>[3x]MKQKLLVTLLGLSALGASPVFAANTNVDLAEDAYIYGYSIDEAYKFFYHTAVENNYPLNEFQNRRALADDSYTAHPTINNDTLHLMGWLDVAAEPVIVSVPDMDEGRYWILHTMDMGHYTNAAFSSRTRGTKGGQFMFAAQDWQGEVPASVDEVV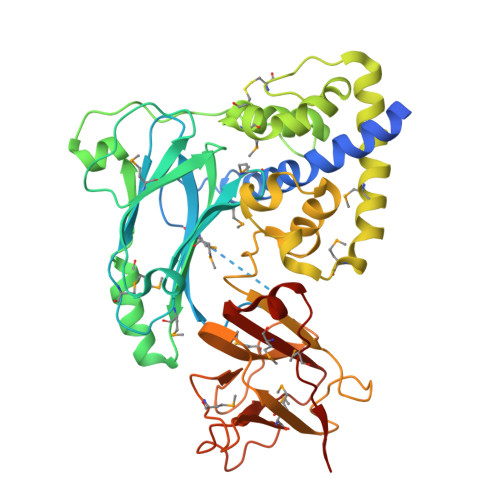RVDSNLVKLMGRIMAVNDEDAKVALNYMDQWNIRTLSEYLGKNGPKPVQRTYPDPKKSTWLERVNFVLCDGSMGNADKQWLDKYQSIGVEPCKTDFTPEQLKLAKVGEKKGMEHLVELAPKMTDARTLLGTRDTLGDAPRDIFAEGTYLGQWGLPPIEASYRKSDFDSIGQKLDGSKHDYVMRFKAPNVSEFWSVTIYGNDNRLMAKNDLNRHSRGDRTMKADKDGYYTIYMSANEKGRADDPNFLPVPEKPFYAIMRFYGADDAIQSGEYQMPEIKVVKLEHHHHHH> ILGGREAEAHARPYMASVQLNGAHLCGG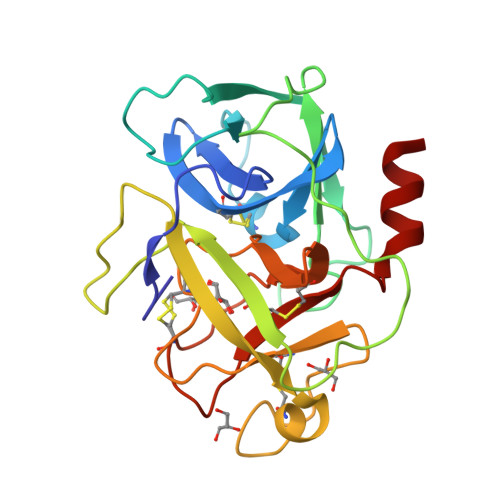VLVAEQWVLSAAHCLEDAADGKVQVLLGAHSLSQPEPSKRLYDVLRAVPHPDSQPDTIDHDLLLLQLSEKATLGPAVRPLPWQRVDRDVAPGTLCDVAGWGIVNHAGRRPDSLQHVLLPVLDRATCNRRTHHDGAITERLMCAESNRRDSCKGDAGGPLVCGGVLEGVVTSGSRVCGNRKKPGIYTRVASYAAWIDSVLA>MASMKVAVLPGDGIGPEVTEAALKVLRALDEAEGLGLAYEVFPFGGAAIDAFGEPFPEPTRKGVEEAEAVLLGSVGGPKWDGLPRKIRPETGLLSLRKSQDLFANLRPAKVFPGLERLSPLKEEIARGVDVLIVRELTGGIYFGEPRGMSEAEAWNTERYSKPEVERVARVAFEAARKRRKHVVSVDKANVLEVGEFWRKTVEEVGRGYPDVALEHQYVDAMAMHLVRSPARFDVVVTGNIFGDILSDLASVLPGSLGLLPSASLGRGTPVFEPVHGSAPDIAGKGIANPTAAILSAAMMLEHAFGLVELARKVED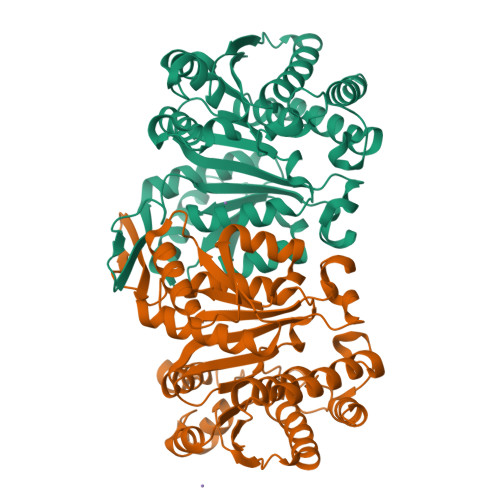AVAKALLETPPPDLGGSAGTEAFTATVLRHLAAAALEHHHHHH[2x]>MRESGWKLIDPISDFGRMGIPNRNWTITDANRNYEICSTYPPEIVVPKSVTLGTVVGSSKFRSKERVPVLSYLYKENNAAICRCSQPLSGFYTRCVDDELL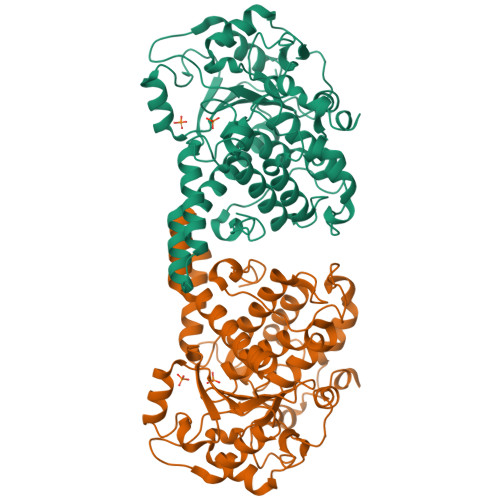LEAISQTNPGSQFMYVVDTRPKLNAMANRAAGKGYENEDNYANIRFRFMGIENIHVMRSSLQKLLEVCELKTPTMSEFLSGLESSGWLRHIKAIMDAGIFITKAVKVEKASVLVHSSDGWDRTAQVCSVASILLDPFYRTFKGLMILIEKEWISMGHKFSQRCGHLDGDSKEVSPIFTQFLDCIWQLMEQFPCAFEFNENFLLEIHDHVFSCQFGNFLGNCQKDREDLRVYEKTHSVWPFLVQRKPDFRNPLYKGFTMYGVLNPSTVPYNIQFWCGMYNRFDKLEHHHHHH[2x]7N-METHYL-8-HYDROGUANOSINE-5'-DIPHOSPHATE 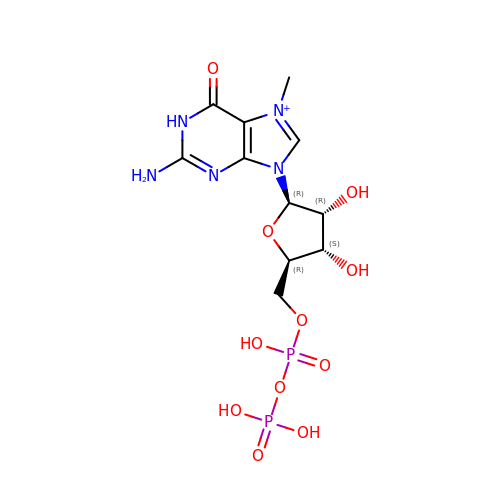| C11 H18 N5 O11 P2 | SBASPRRECYVBRF-KQYNXXCUSA-O> MDNFNYKNDTKIIFGKDNYSEIGKNIKIFSKKTPKILLHYEADGELIKKLGIYEKVISSLKEFDIEFIELGGVVPNPRLSLVYE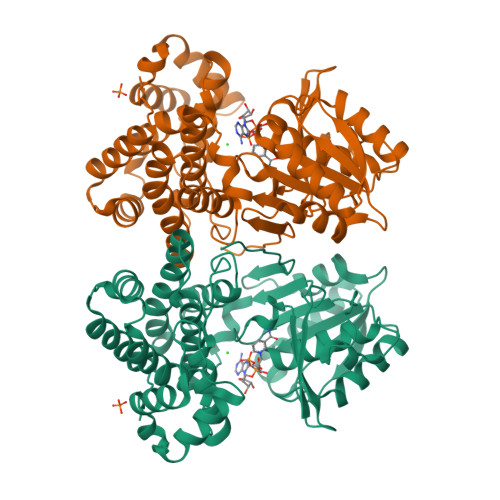GIKICKEENITFILAVGGASVIDSAKAISLGAVDNGDVWDFFTAKRIPQDTLGIGVVLTIPGAGSEMSESSIITDENKKQKAVCDTEVNFPKFAILNPEVCYTIPDRLMAAGIVDILSHLMERYFTKSIDTALSDSLIEATMKIVIKYGPLLMKDRKNYNYCSQIMWAATMAHNGMIACGRVADWASHRIEHEISGIYDLTHGIGMAIIFPAWMKYTKNIRPQIFEKFFKEVFNTVNIDEGINKLEEFFKSLGINLKLSDYGITEEYFSLMAEKALGNSETLGRFMQLNKQDIINILNLAK>[2x]MEEYMPTEHHHHHHENLYFQGTSGEGQDIWDMLDKGNPFQFYLTRVSGVKPKYNSGALHIKDILSPLFGTLVSSAQFNYCFDVDWLVKQYPPEFRKKPILLVHGDKREAKA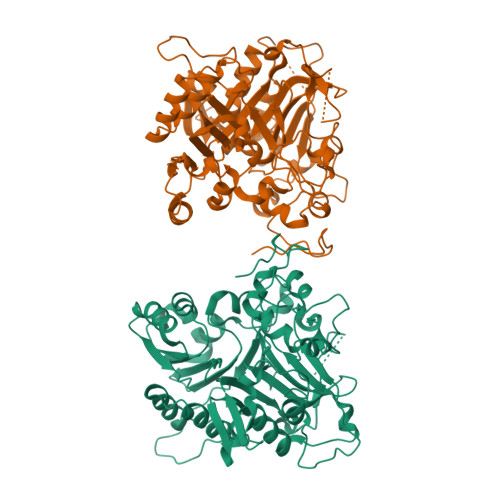HLHAQAKPYENISLCQAKLDIAFGTHHTKMMLLLYEEGLRVVIHTSNLIHADWHQKTQGIWLSPLYPRIADGTHKSGESPTHFKADLISYLMAYNAPSLKEWIDVIHKHDLSETNVYLIGSTPGRFQGSQKDNWGHFRLKKLLKDHASSMPNAESWPVVGQFSSVGSLGADESKWLCSEFKESMLTLGKESKTPGKSSVPLYLIYPSVENVRTSLEGYPAGGSLPYSIQTAEKQNWLHSYFHKWSAETSGRSNAMPHIKTYMRPSPDFSKIAWFLVTSANLSKAAWGALEKNGTQLMIRSYELGVLFLPSAFGLDSFKVKQKFFAGSQEPMATFPVPYDLPPELYGSKDRPWIWNIPYVKAPDTHGNMWVPS In response to environmental stimuli, the bacterium produces and secretes its main virulence factor, the cholera toxin (CT). CT is an AB5 protein toxin, which consists of one toxic A-subunit (CTA) and five identical B-subunits arranged in a doughnut-shaped ring (CTB). The primary receptor of the cholera toxin is the GM1 ganglioside, which is expressed in distinct membrane microdomains of small-intestinal epithelial cells. There are two major biotypes of V. cholerae, classical and El Tor, which produce cholera toxins with a slight sequence variation (cCT and ET CT). cCT and ET CT differ in only two residues of the B-subunit, His18/Tyr18 and Thr47/Ile47 (classical/El Tor).

Moreover, no previous toxin structure has been reported in complex with the blood group H determinant, which is characteristic of blood group O. The crystal structures of the cCTB and ET CTB complexes were determined to a resolution of 1.1 Å and 1.5 Å, respectively. Both proteins crystallized using the same conditions, but in different space groups (P212121 and P21). Well-defined electron density is present in all ten binding sites of the two pentamers, although the ligand orientations differ. While the electron density of the cCTB structure primarily supports orientation 2, most ET CTB binding sites exhibit the ligand in orientation 1. Since H-tetra-BGA is an almost symmetrical molecule, the fucosyl residues are indistinguishable. As for the complexes with A-penta-BGA, the fucose near residue 47 is most tightly anchored to the toxin, while the other fucose is loosely bound, by indirect water-mediated interactions. In general, the two structures are very similar, except that the N-acetyl group changes place in the two different orientations; the axial 4-OH group of Gal is mimicked by the α-anomer of GlcNAc. In addition to the ligands at the secondary binding site, the two structures of cCTB contain Gal monosaccharides in the primary binding site, which shows that the toxin can bind ligands at both binding sites simultaneously. Galactose is presumably a remnant from the purification by D-Gal affinity chromatography.

>[10x]TPQNITDLCAEYHNTQIHTLNDKIFSYTESLAGKREMAIITFKNGATFQVEVPGSQHIDSQKKAIERMKDTLRIAYLTEAKVEKLCVWNNKTPHAIAAISMAN>[3x]MAHNNENVSGISAYL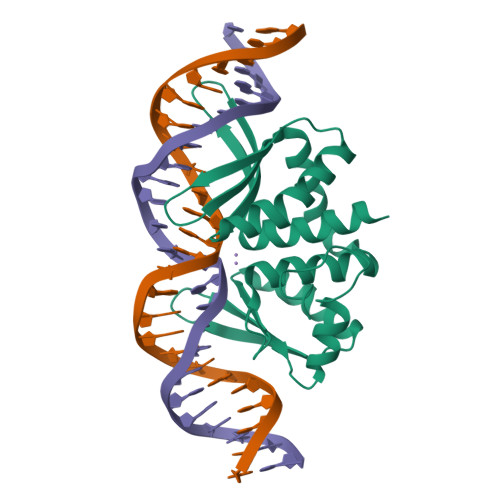LGLIIGDGGLYKLKYKGNRSEYRVVITQKSENLIKQHFAPLMQFLIDELNVKSKIQIVKGDTRYELRVSSKKLYYYFANMQERIRLFNMREQIAFIKGLYVAEGDKTLKRLRIWNKNKALLEIVSRWLNNLGVRNTIHLDDHRHGVYVLNISLRDRIKFVHTILSSHLNPLPPEAAALEHHHHHH>GPAVRTIRIYQPGEYQPGQLLELSPEAGQHVGVVLRMEQGEQLTLFNGDNKEFTASIERVKKKQVFVRIASVLEVNRESPLKIHLAQAISKGERMEMVMQKSAELGVACITPLITERCQVKIDKEKMAKKMHQWLNIIIGACEQCGRNQIPELRQPVYLDQFVREAKEHLKLILHPAFSKTWRDYPVQPPDVALIIGPEGGFSDEEIRLTSGHGFLPLSLGPRVLRTETAAITALSVLQAAGGDL[8x]

The methylation of U1498 located in the 16S ribosomal RNA of Escherichia coli is an important modification affecting ribosomal activity. RsmE methyltransferases methylate specifically this position in a mechanism that requires an S‐adenosyl‐L‐methionine (AdoMet) molecule as cofactor. The protein comprises an N‐terminal PUA domain and a C‐terminal SPOUT domain. The latter is responsible for protein dimerization and cofactor binding.

Here we report the structure of Apo and AdoMet‐bound Lpg2936 from Legionella pneumophila at 1.5 and 2.3 Å, respectively. Comparison with similar structures suggests that Lpg2936 is an RsmE‐like enzyme that can target the equivalent of U1498 in the L. pneumophila ribosomal RNA, thereby potentially enhancing ribosomal activity during infection‐mediated effector production. The multiple copies of the enzyme found in both structures reveal a flexible conformation of the bound AdoMet ligand. Isothermal titration calorimetry measurements suggest an asymmetric two site binding mode. Our results therefore also provide unprecedented insights into AdoMet/RsmE interaction, furthering our understanding of the RsmE catalytic mechanism.(2R,15R)-2-[(1-aminoisoquinolin-6-yl)amino]-4,15,17-trimethyl-7-[1-(1H-tetrazol-5-yl)cyclopropyl]-13-oxa-4,11-diazatricyclo[14.2.2.1~6,10~]henicosa-1(18),6(21),7,9,16,19-hexaene-3,12-dione 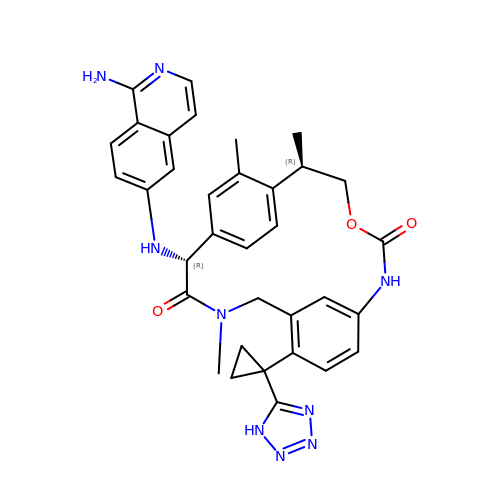| C34 H35 N9 O3 | YSEANFNTDGIIGS-AFJIDDCJSA-N>[2x]DYKDDDDKGSSSSNVEVFIPVSQGNTNGFPATASNDLKAFTEGAVLSFHNICYRVKLKSGFLPCRKPVEKEILSNINGIMKPGLNAILGPTGGGKSSLLDVLAARKDPSGLSGDVLINGAPRPANFKCNSGYVVQDDVVMGTLTVRENLQFSAALRLATTMTNHEKNERINRVIQELGLDKVADSKVGTQFIRGVSGGERKRTSIGMELITDPSILFLDEPTTGLDSSTANAVLLLLKRMSKQGRTIIFSIHQ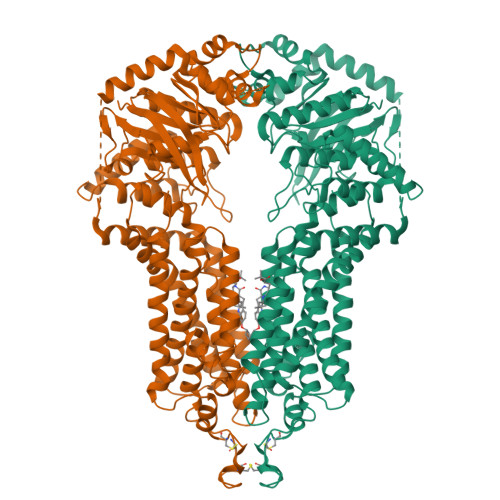PRYSIFKLFDSLTLLASGRLMFHGPAQEALGYFESAGYHCEAYNNPADFFLDIINGDSTAVALNREEDFKATEIIEPSKQDKPLIEKLAEIYVNSSFYKETKAELHQLSGGEKKKKITVFKEISYTTSFCHQLRWVSKRSFKNLLGNPQASIAQIIVTVVLGLVIGAIYFGLKNDSTGIQNRAGVLFFLTTNQCFSSVSAVELFVVEKKLFIHEYISGYYRVSSYFLGKLLSDLLPMRMLPSIIFTCIVYFMLGLKPKADAFFVMMFTLMMVAYSASSMALAIAAGQSVVSVATLLMTICFVFMMIFSGLLVNLTTIASWLSWLQYFSIPRYGFTALQHNEFLGQNFCPGLNATGNNPCNYATCTGEEYLVKQGIDLSPWGLWKNHVALACMIVIFLTIAYLKLLFLKKYS> QDAKAGEAVFKQCMTCHR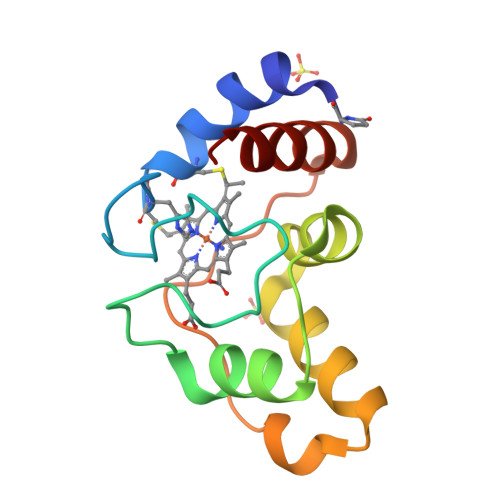ADKNMVGPALAGVVGRKAGTAAGFTYSPLNHNSGEAGLVWTADNIVPYLADPNAFLKKFLTEKGKADQAVGVTKMTFKLANEQQRKDVVAYLATLK> GLEDCDFGWSPYDQHCYQAFNEQKTWDEAEKFCRAQENGAHLASIESNGEADFVSWLISQKDELADEDYVWIGLRAQNKEQQCSSEWSDGSSVSYENLIDLHTKKCGALEKLTGFRKWVNYYCEQMHAFVCKLLPY;> DCPSGWSSYEGHCYKPFNEPKNW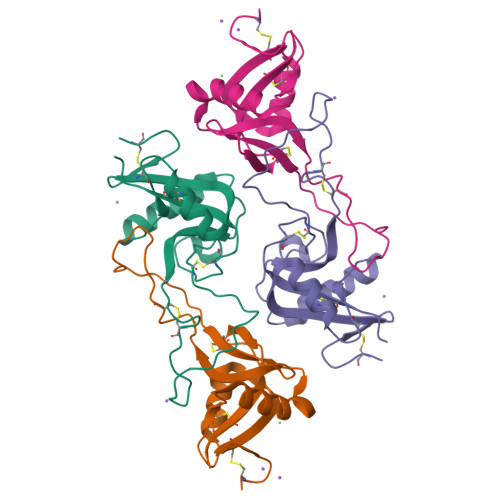ADAERFCKLQPKHSHLVSFQSAEEADFVVKLTRPRLKANLVWMGLSNIWHGCNWQWSDGARLNYKDWQEQSECLAFRGVHTEWLNMDCSSTCSFVCKFKA> MHHHHHHSSGRENLYFQGHMETSVPPGSALVGPSCVMDDFRDPQRWKECAKQGKMPCYFDLIEENVYLTERKKNKSHRDIKRMQCECTPLSKDERAQGEIACGEDCLNRLLMIECSSRCPNGDYCSNRRFQRKQHADVEVILTEKKGWGLRAAKDLPSNTFVLEYCGEVLDHKEFKARVKEYARNKNIHYYFMALKNDEIIDATQKGNCSRFMNHSCEPNCETQKWTVNGQLRVGFFTTKLVPSGSELTFDYQFQRYGKEAQKCFCGSANCRGYLGGENRVSIRAAGGKMKKERSRK;> APATGGVMKPHRYRP

In this study, we solved the structures of an H3K36M peptide in complex with the catalytic SET domain of mammalian SETD2 and S-adenosylmethionine (SAM), or S-adenosyl-L-homocysteine (SAH), and revealed the detailed molecular mechanism by which SETD2 interacts with the histone H3 tail. NSD1, NSD2/MMSET, NSD3, and ASH1L are responsible for H3K36me2 and H3K36me1, whereas SETD2 is responsible for H3K36me3. In addition, the enzymatic activity of SETD2 is inhibited by the H3K36M mutation, and SETD2 failed to methylate histone tails containing H3G34 mutations, making it ideal to further study the molecular mechanisms of oncogenic histone mutations in regulating H3K36 methylation. To understand the molecular details of the interactions, we generated recombinant SET domain of SETD2 (residue 1435–1711, encompassing the AWS, SET, and post-SET regions) and an H3K36M peptide (29-APATGGVMKPHRYRP-43).

We then determined the 2.42 Å resolution crystal structure of the SET domain of SETD2 in complex with the H3K36M peptide and SAM. Clear electron density was observed for the entire H3K36M peptide and SAM based on the crystallographic analysis. Residues 32–43 of the peptide assume an extended conformation, and residues 33–35 have anti-parallel interaction with a strand (residues 1668–1670) in the post-SET motif of SETD2. The K36M residue of histone H3 is located in the active site of SETD2, confirmed by the fact that a doubly methylated lysine residue (Mly9) of the H3K9 peptide is bound at a similar position in the SET domain of its methyltransferase GLP-1. The methionine side chain does not extend as deeply into the pocket as compared to the lysine side chain. It is surrounded by a collection of aromatic side chains (Tyr1579, Tyr1605, Phe1650, Phe1664, Tyr1666, Phe1668) as well as Met1607 from SETD2. The methyl group of the cofactor SAM is pointed toward the K36M side chain of the peptide, but at a distance of 4.2 Å to its sulfur atom and 4.3 Å to its methyl group, suggesting it does not directly mediate interaction with the methionine side chain. Therefore, the contribution of SAM to the interaction between SETD2 and H3K36M is mainly to stabilize the proper folding of the SET domain. Our structural data indicated that the electron density for the methyl group is weaker compared to the rest of SAM, suggesting that a mixture of SAM and SAH are present in this structure. As we only added SAM during crystallization, SAH is likely a degradation product, as has been observed before. In fact, our SETD2-H3K36M-SAM structure showed that the methyl group of SAM has a lower electron density, most likely due to the degradation of SAM during crystallization.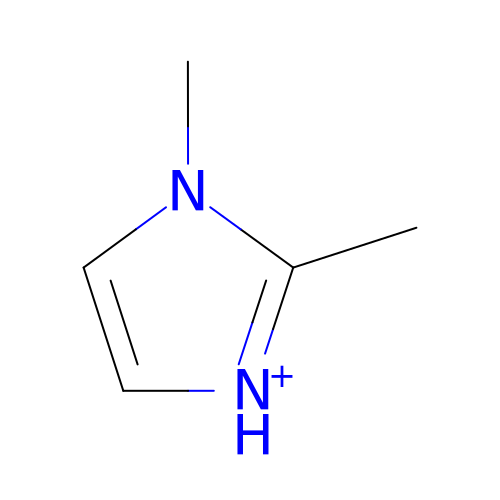2,3-DIMETHYLIMIDAZOLIUM ION | C5 H9 N2 | GIWQSPITLQVMSG-UHFFFAOYSA-O>[2x]SAPVRLPFSGFRLQKVLRESARDKIIFLHGKVNEASGDGDGEDAVVILEKTPFQVEQVAQLLTGSPELQLQFSNDIYSTYHLFPPRQLNDVKTTVVYPATEKHLQKYLRQDLRLIRET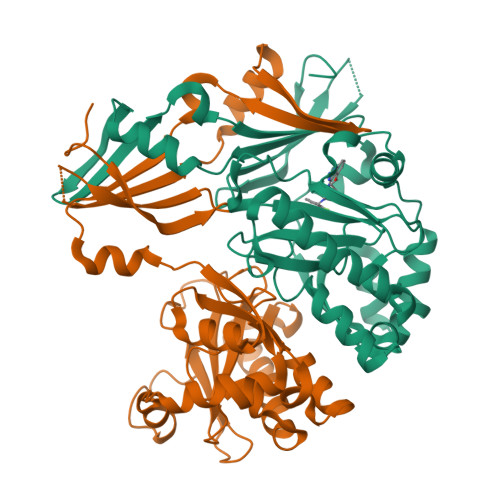GDDYRNITLPHLESQSLSIQWVYNILDKKAEADRIVFENPDPSDGFVLIPDLKWNQQQLDDLYLIAICHRRGIRSLRDLTPEHLPLLRNILHQGQEAILQRYRMKGDHLRVYLHYLPSYYHLHVHFTALGFEAPGSGVERAHLLAEVIENLECDPRHYQQRTLTFALRADDPLLKLLQEAQQS> MAEPKAQGTQKVESSTTKKEVKDAEETIKIPTLEDIDNLIDSAEEVKSEEDINKMPPLKFPVEFPEVNTRSIIGGNNYPIVLVHGFMGFGRDELLGYKYWGGVVDLQEKLNASGHETYTATVGPVSSNWDRACELYAYIVGGTVDYGEAHAKKFKHNRYGRTYPGIYKNISNENKIHLIGHSMGGQTIRTLTQLLSEGSEEEINCGQENISPLFEGGKHWIHSVSTISTPNDGTTLSDLMPAKDLISYTFGVLGTITGKNKLFSSIYDLKLDQWGLKKQNGESQRDYIERVLDSNIWNSTKDIATYDLSTEGAQELNTWVKAQPDVYYFSWTTQATKESILTGHSVAQIGPMNPIFYPTANLMGRYSRNQKDLPIIDKKWFPNDGVVNCISQDGPKLGSNDVIEQYNGGVKIGQWNAMPRIINTDHMDIVGTFGNVKDWYMDYASFLSNLSRALE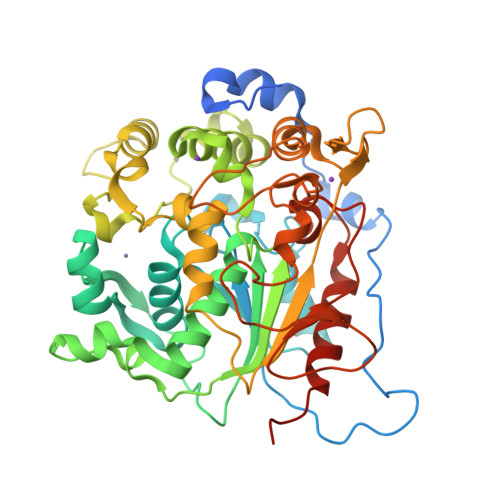HHHHHH>[2x]AVSKVYARSVYDSRGNPTVEVELTTEKGVFRSIVPSGASTGVHEALEMRDGDKSKWMGKGVLHAVKNVNDVIAPAFVKANIDVKDQKAVDDFLISLDGTANKSKLGANAILGVSLAASRAAAAEKNVPLYKHLADLSKSKTSPYV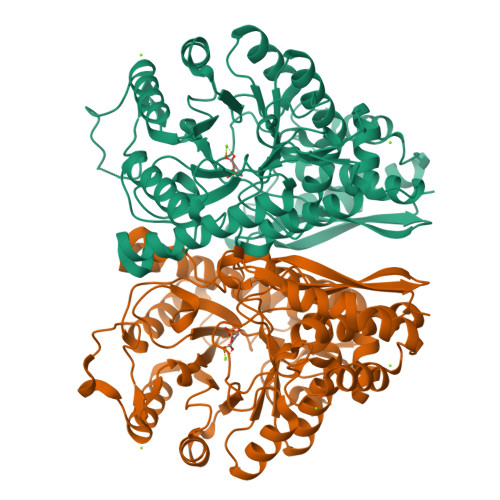LPVPFLNVLNGGSHAGGALALQEFMIAPTGAKTFAEALRIGSEVYHNLKSLTKKRYGASAGNVGDEGGVAPNIQTAEEALDLIVDAIKAAGHDGKIKIGLDCASSEFFKDGKYDLDFKNPNSDKSKWLTGPQLADLYHSLMKRYPIVSIEDPFAEDDWEAWSHFFKTAGIQIVADALTVTNPKRIATAIEKKAADALLLKVNQIGTLSESIKAAQDSFAAGWGVMVSHRSGETEDTFIADLVVGLRTGQIKTGAPARSERLAKLNQLLRIEEELGDNAVFAGENFHHGDKLLHHHHHH>GSAKDPMKRESNIQVLSRGQKDQPVSQIYQVSTMTSLLDGVYDGDFELSEIPKYGDFGIGTFNKLDGELIGFDGEFYRLRSDGTATPVQNGDLSPFCSFTFFTPDMTHKIDAKMTREEFEKEINSILPSKNLFYAIRIDGLFKKVQTRTVELQEKPYVPMVEAVKTQPIFNFDNVRGTIVGFLTPAYANGIAVSGYHLHFIDEGRNSGGHVFDYVLEDCTVTISQKMNMNLRLPNTADFFNANLDN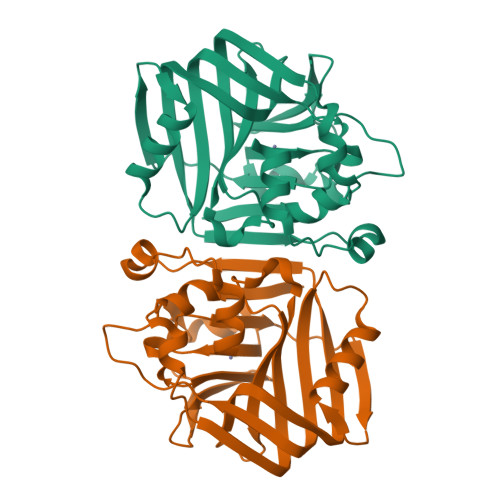PDFAKDIETTEGSPE[2x]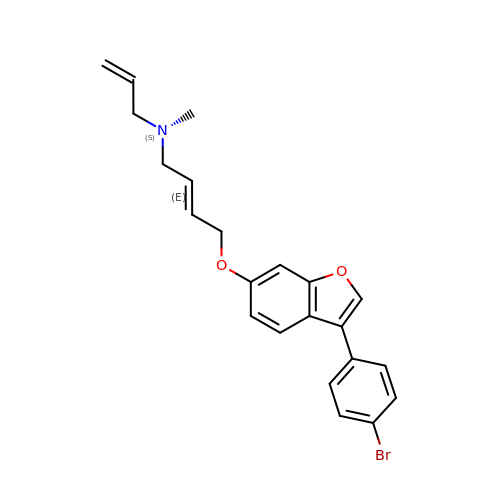ALLYL-{4-[3-(4-BROMO-PHENYL)-BENZOFURAN-6-YLOXY]-BUT-2-ENYL}-METHYL-AMINE | C22 H22 Br N O2 | KCNKJCHARANTIP-SNAWJCMRSA-N> MVKKKEPAEGWPVVSGDYIVGDPESPVAAVTLASHIEDIPIDAGAAIAGPCKTENLGIEKVIANIISNPNIRFLVLCGSEVQGHIVGQSMKALHKNGVDDKRK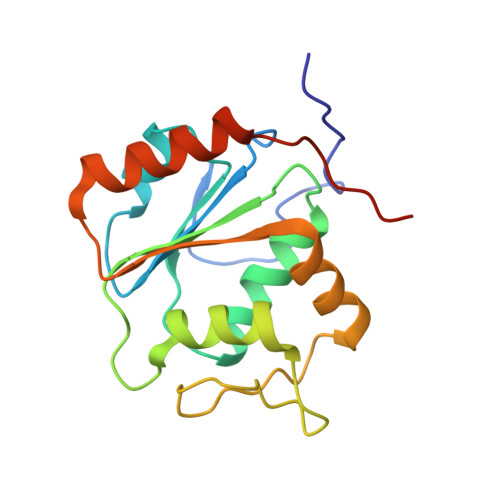IIGAKGAIPYIENLPEEALERFQKQVEIVDLIDVEDADQIKEKVKECIEKDPGAFEEEEVILRL> EPGLPPGPLENSSAKLVNDEAHPWKPLRPGDIRGPCPGLNTLASHGYLPRNGVATPAQIINAVQEGFNFDNQAAIFLTYAAHLVDGNLITDLLSIGRKTRLTGPDPPPPASVGGLNEHGTFEGDASMTRGDAFFGNNHDFNETLFEQLVDYSNRFGGGKYNLTVAGELRFKRIQDSI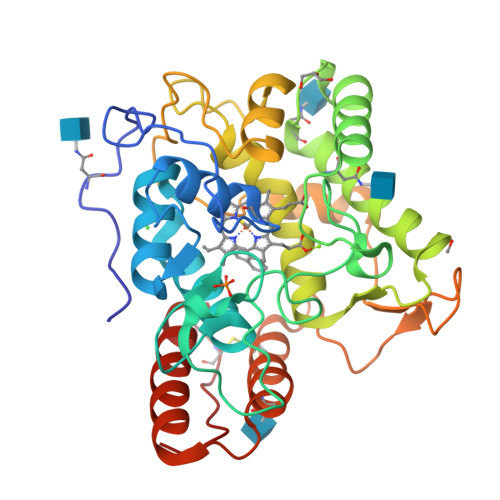ATNPNFSFVDFRFFTAYGETTFPANLFVDGRRDDGQLDMDAARSFFQFSRMPDDFFRAPSPRSGTGVEVVVQAHPMQPGRNVGKINSYTVDPTSSDFSTPCLMYEKFVNITVKSLYPNPTVQLRKALNTNLDFLFQGVAAGCTQVFPYGRD> MADIIASVDKKDVFAVSDTSYFKNFKFPSKKISDTGEVIDSTKLPQIKDTYKSSREEPIPDNDSTINVKNITTYHYLEAQKPKNSSIELTMVAPSKSKKPNDCVVEAINDNNKIYTPFSGTAKQFNTVVPIANTAANVITWLEAIADIFSSETGTFDKLERAGKETLYYIPYVGQLLSIGENVLIGDFKNALLNTGLIILLDIAPELNIPLLGAFEAYKEYKSLEEFRKAIDNVIDERNKRWHSVYSFVAHQWYGQVNIQIEQRLNHFYQALSYQAGVIKNRVDIEYARHKEGLEEKEERKLMWASVDCIGSIEASVKEATKNAEKFLEKSSILYFKEEILPKVHKNLEEFDKNTLFNIYTNIDEFSNRGIAEISECKKVEADVNNGFRPIKFDFSLLTNLMKSDSLTDEVILEKALEDALVFSLGVRNGKIQNLSKKWANLTIGTDIRVVHGRDNESIRLNSTQDSSIQIEKNTNLRFLDSENFSLSFW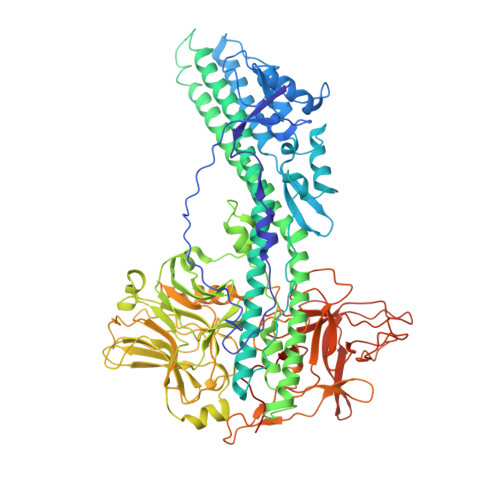IRVPRYNKFDKDKDLNNEYTIVNNMDTATKGFKISIKNGILLWTLKGTQQKTIEIPLSNTKVSDNIWRHVAIINNKDGNCTIYVDGAQKNAVSLSGLDEITNTLPITLQLVGNKNKKQFIRLDQFNIYEKALSQTEVGKLFSSYFKDSDIRDYWGEPLAYNKTYNMINIAYQGRGLQSTNNKISLQPKAVFDPTGDGSYIPRLYRGYDVLLQKDSQSKTTDIMPKKDDLINIKLKSGHNFVGFNSTIDTSQKYLKLTTALLSEVDDPKGFKLMSLKKDNWIQIKKETWMSKNGNVIPQGLVGKRSVDSDVYLYLWDWETEKDDYSEKQWSFICQDEGWIDSDGMFTNA>[8x]MAHHHHHHSPVIHAETTAAPVLENRAAQGDITTPGGARRLTGDQTEALRASLINKPAKNVILLIGDGMGDSEITAARNYAEGA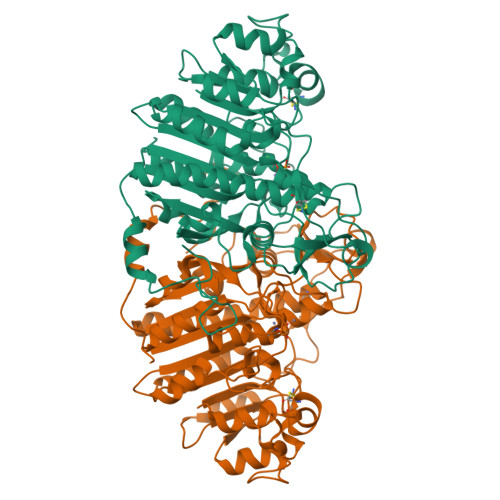GGFFKGIDALPLTGQYTHYSLDKKTGKPDYVTDSAASATAWTTGVKTYNGALGVDIHENAHQTILELAKAAGLATGNVSTAELQDATPAALVAHVTSRKCYGPTVTSEKCPSNALEKGGKGSITEQLLNARPDVTLGGGAKTFAETATAGEWQGKTLREQAQARGYQIVTDAASLAAATEASQDKPLLGLFADGNMPVRWEGPKASYHGNIDKPPVTCTPNPKRDASVPTLAQMTEKAIDLLSRNEKGFFLQVEGASIDKQDHAANPCGQIGETVDLDEAVQKALEFARKDGNTLVIVTADHAHASQIIPADSKAPGLTQALNTHDGAVMVMSYGNSEEESMEHTGTQLRIAAYGPHAANVVGLTDQTDLFTTMKAALSLK>MLTVDLSGKKALVMGVTNQRSLGFAIAAKLKEAGAEVALSYQAERLRPEAEKLAEALGGALLFRADVTQDEELDALFAGVKEAFGGLDYLVHAIAFAPREAMEGRYIDTRRQDWLLALEVSAYSLVAVARRAEPLLREGGGIVTLTYYASEKVVPKYNVMAIAKAALEASVRYLAYELGPKGVRVNAISAGPVRTVAARSIPGFTKMYDRVAQTAPLRRNITQEEVGNLGLFLLSPLASGITGEVVYVDAGY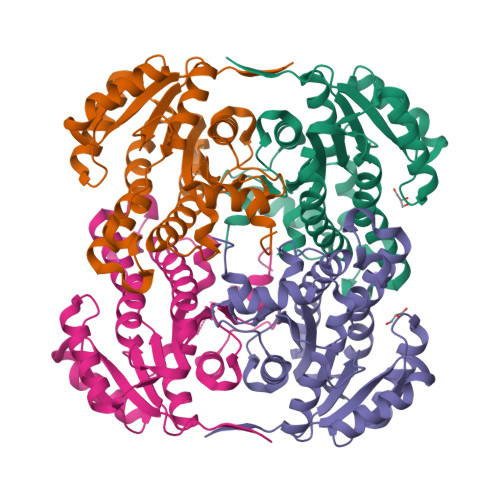HIMGMELEG[4x]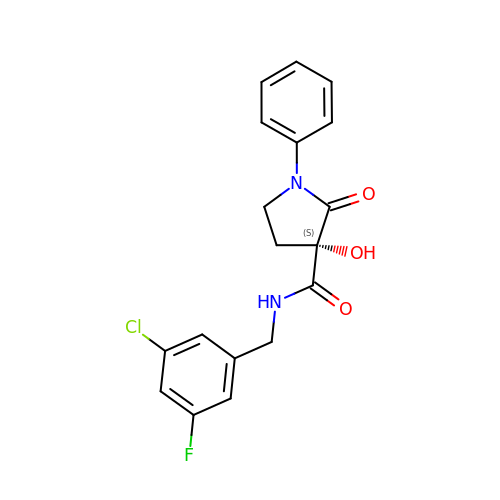(3~{S})-~{N}-[(3-chloranyl-5-fluoranyl-phenyl)methyl]-3-oxidanyl-2-oxidanylidene-1-phenyl-pyrrolidine-3-carboxamide | C18 H16 Cl F N2 O3 | GYXUHDDOWYYRFT-SFHVURJKSA-N>[2x]MKNTIHINSNDSVTLRLMTEHDLAMLYEWLNRSHIVEWWGGEEARPTLADVQEQYLPSVLA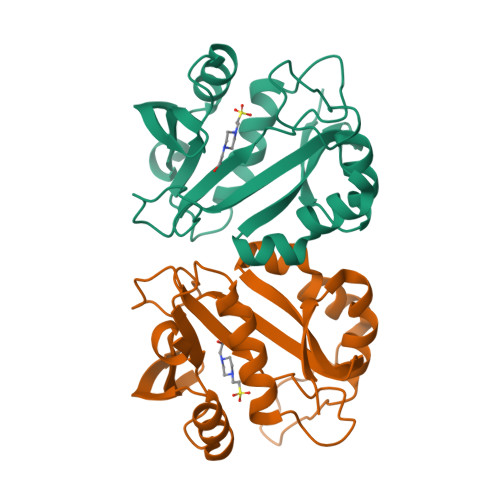QESVTPYIAMLNGEPIGYAQSYVALGSGDGWWEEETDPGVRGIDLSLANASQLGKGLGTKLVRALVELLFNDPEVTKIQTDPSPSNLRAIRCYEKAGFERQGTVTTPDGPAVYMVQTRQAFERTRSDEGRAQFEA(2S)-2-hydroxy-2-methyl-N-[4-nitro-3-(trifluoromethyl)phenyl]-3-(pentafluorophenoxy)propanamide 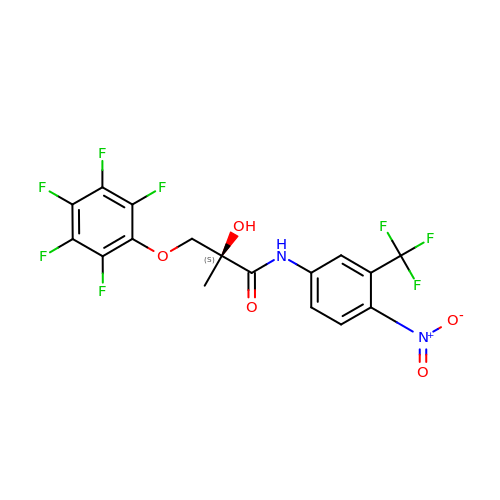| C17 H10 F8 N2 O5 | MMNRWNREMUMYQG-INIZCTEOSA-N>[2x]LEQYVKKILTSRVYDVAVETPLQPARQLSERLGNQVLLKREDLQPVFSFKIRGAYNKVAQLTEEEKARGVIAASAGNHAQGLALAAKRQGIRAVIVMPKTTPEIKVQAVRAHGAKAVLHGDAFPEALAHALKLVDEKGYTFVHPYDDPDTIAGQGTVAMEILRQQPGRLDAIFVPVGGGGLVAGIAAYVKYLRPEIKVIGVEPDESNCLQAAMAAGERVVLGQVGLFADGVAVAQIGQHTFDICKDHVD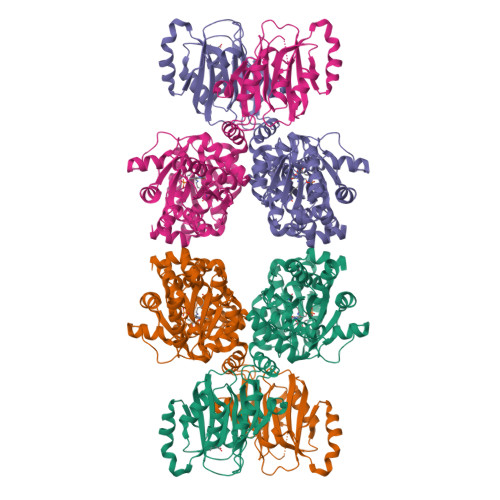EVITVSTDEICAAIKDIYDDTRSITEPAGALAVAGIKKYVERERAEGQTLVAIDSGANVNFDRLRHVAERAELGERREAIIAVTIPERPGSFKAFCEAVGKRQITEFNYRYHSGSEAHIFVGVQTHPENDPREALVAYLREKGFPVLDLTDNELAKLHIRHMVGGHAVKVSDEMVFRFEFPERPGALFNFLTKLGGRWNISMFHYRNHGAADGRVVAGLQVPEDERHLIPQTLEAIGYPYWDETANPAYQLFL>SNAMKTYKVAVLAGDGIGPLVMKEALKILTFIAQKYNFSFELNEAKIGGASIDAYGVALSDETLKLCEQSDAILFGSVGGPKWDNLPIDQRPERASLLPLRKHFNLFANLRPCKIYESLTHASPLKNEIIQKGVDILCVRELTGGIYFGKQDLGKESAYDTEIYTK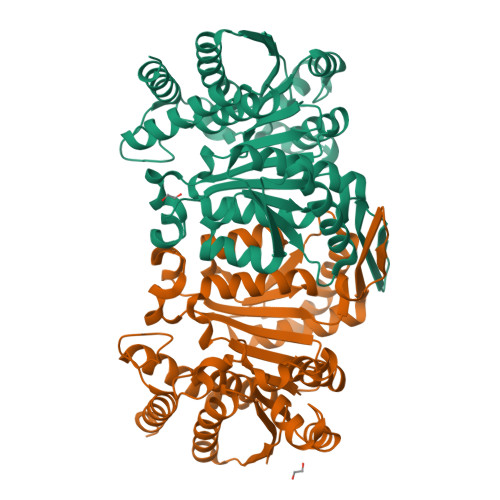KEIERIARIAFESARIRKKKVHLIDKANVLASSILWREVVANVAKDYQDINLEYMYVDNAAMQIVKNPSIFDVMLCSNLFGDILSDELAAINGSLGLLSSASLNDKGFGLYEPAGGSAPDIAHLNIANPIAQILSAALMLKYSFKEEQAAQDIENAISLALAQGKMTKDLNAKSYLNTDEMGDCILEILKENDNG[8x]>[2x]GSHMSVDLDPSARFAEYAHPERLVSTEWLAAHLGDEGLVVVESDEDVLLYETGHIPGAVKVDWHTDLNDPVQRDYIDGAAFAALLGERGISRDTTVVIYGDKNNWWAAYALWVFTLFGHDDVRLLDGGRSKWEAEGRAYTTDAPTVAATSYPVVERDDSRIRAYRDDVLAHFGKPLIDVRSPEEFSGARTTAPAYPEEGALRAGHIPSAQNVPWGKAAAEDGTFRTLAELDALYRDGAGLKDGDDVVAYCRIGERSSHTWFVLQHLLGFENVRNYDGSWTEWGSAVRVPIVQGSEPGEAPAPIVGR

Sulfurtransferases, also known as rhodaneses, facilitate the transfer of sulfur from a donor molecule to a thiophilic acceptor. FrST exists as a dimer and can be classified as a TST rather than an MST according to sequence-based clustering and enzyme activity. Each subunit of FrST comprised 11 α-helices, two 310 helices, and six β-strands and was divided into two distinct domains: the N-terminal rhodanese fold domain (non-active domain) and the C-terminal rhodanese fold domain (active domain). The active site of FrST was composed of Trp102, Val176, Arg177, Glu181, Trp211, Arg248, and Arg252, which surrounded catalytic Cys247.

Within the crystal, each asymmetric unit contained two subunits, designated A and B. After refinement, the final protein model of FrST exhibited a crystallographic R-factor of 23% and a free R-factor of 26%. The model comprised 302 residues and 339 water molecules. However, the remaining residues were successfully traced based on the electron density, except for a loop of Thr188–Glu194 (later termed as 8α-η2 loop region) in subunit B, indicating the high flexibility of this loop region. During the crystal structure determination, we also solved another crystal structure of FrST, which belongs to the I21 space group and is annotated as FrSTI21. The overall structure of both structures is almost identical, evidenced by an RMSD of 0.284 Å (Cα). However, when FrSTI21 could closely resemble FrSTP1, a distinct conformational difference was observed in the 8α-η2 loop region at the top of the active site. In subunit A of FrSTP1, the 8α-η2 loop region (residues Ala186–Ala198) adopted an open conformation, as supported by clear electron density in the corresponding map. Glu195 formed hydrogen bonds with Arg248 and Arg252 from the active site loop, while Tyr192 interacted with neighboring Arg252 through a cation-π interaction. Volume analysis using ParKVFinder 3.0 revealed that the volume of the active site in FrSTP1was 8.2 Å3, whereas it was 12.3 Å3 in FrSTI21. The diverse amino acid composition and structural flexibility, as evidenced by weak electron density in the 8α-η2 loop region, suggests that this region is likely involved in an open and closed mechanism that facilitates substrate recognition and selectivity.> QAQIT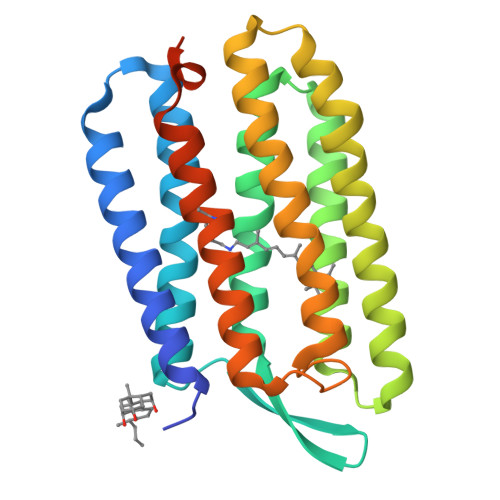GRPEWIWLALGTALMGLGTLYFLVKGMGVSDPDAKKFYAITTLVPAIAFTMYLSMLLGYGLTMVPFGGEQNPIYWARYADWLFTTPLLLLDLALLVDADQGTILALVGADGIMIGTGLVGALTKVYSYRFVWWAISTAAMLYVLYVLFFGFTSKAESMRPEVASTFKVLRNVTVVLWSAYPVVWLIGSEGAGIVPLNIETLLFMVLDVSAKVGFGLILLRSRAIFGEAEAPEPSAGDGAAATSD> GSHMDSLRPKLSEEQQRIIAIL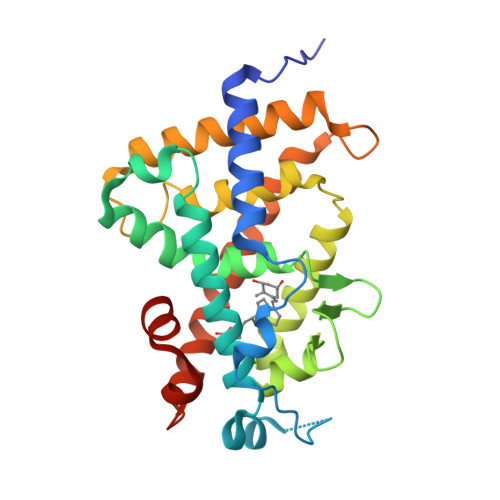LDAHHKTYDPTYSDFCQFRPPVRVNDGGGSVTLELSQLSMLPHLADLVSYSIQKVIGFAKMIPGFRDLTSEDQIVLLKSSAIEVIMLRSNESFTMDDMSWTCGNQDYKYRVSDVTKAGFSLELIEPLIKFQVGLKKLNLHEEEHVLLMAICIVSPDRPGVQDAALIEAIQDRLSNTLQTYIRCRHPPPGSHLLYAKMIQKLADLRSLNEEHSKQYRCLSFQPECSMKLTPLVLEVFGNEIS2-(trifluoromethyl)-9~{H}-purine-6-thiol | C6 H3 F3 N4 S | 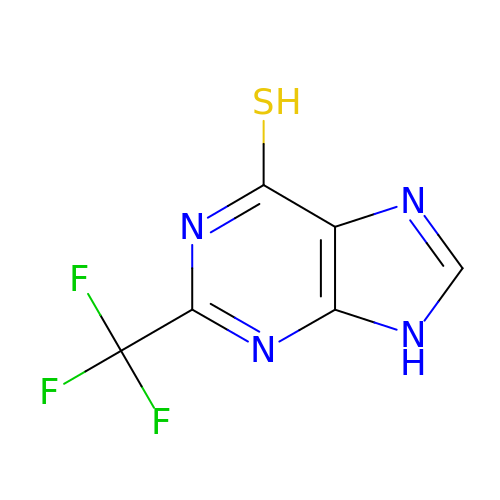NVRHELPZQYUXMX-UHFFFAOYSA-N>GSMTTVMNDKHPTPDPAEDNAFFPSAYSLSQFTASKSDLSGAHYPTPYQGGRWKILVVGADERYLMMDNGTFFSTGNHPVETLLPMYHLDKAGFSFDIATLSGNPVKFEWWAMPREDQEVNGLYSKYQSSFRQPLKLSDVIETALGEDSDYIGVFIPGGHGALMGLPDSQEVKAVLQWAMKQNKFIISLCHGPAAFLAVGDDPLFAGYKIVAFPDEMDAQTPSIGYMPGHLTWKFGE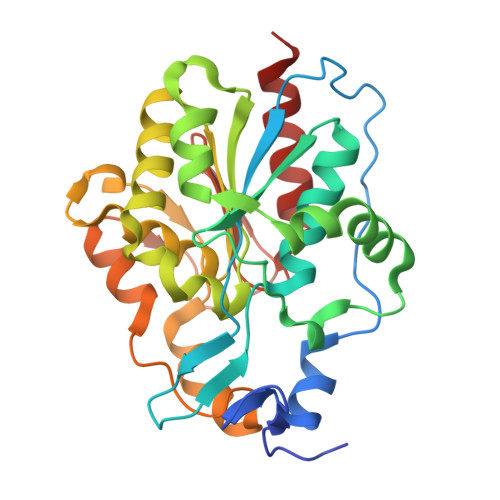QLQAIGFELLNTGISGQVFQDRKMLTGDSPLAGNALGQLAAKALLAEVEQK[6x]2-[6-(cyclobuta-1,3-dien-1-ylamino)-1,3-benzothiazol-2-yl]-1,3-thiazol-4-ol 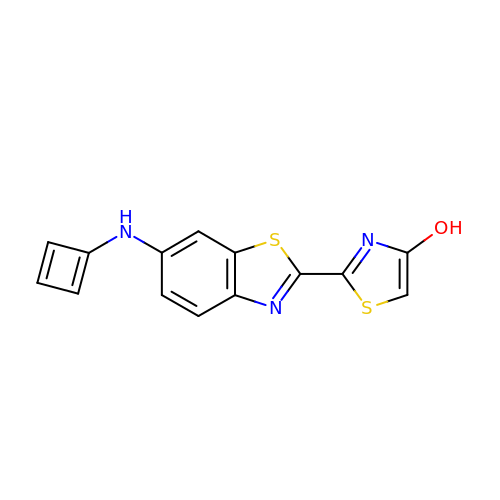| C14 H9 N3 O S2 | AMUPGDQXMKYKJQ-UHFFFAOYSA-N(2S,4aR,6R,7R,7aS)-6-{6-amino-8-[(4-fluorobenzyl)sulfanyl]-9H-purin-9-yl}-2-sulfanyltetrahydro-4H-furo[3,2-d][1,3,2]dioxaphosphinin-7-ol 2-oxide | C17 H17 F N5 O5 P S2 | 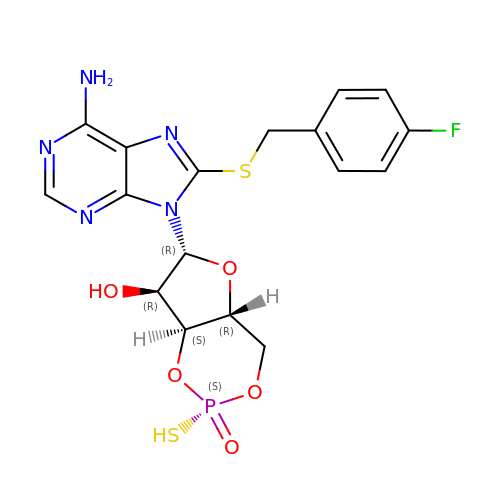HQPHMVRGPVFPCD-BVGSDMBWSA-N>MEQYSEACIEACIDCMKACNHCFTKCLEESVQHHLSGCIRLDRECADICALAVKAMQTDSPFM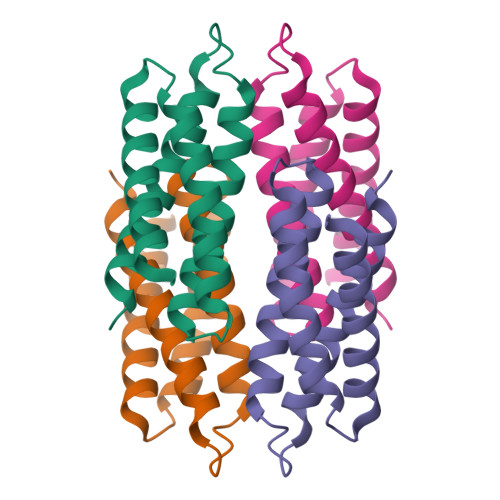KEICALCADICEACGTECGKHDHDHCQACAKACFTCAEQCRSMAA[4x]>MSLRYIVALTGGIGSGKSTVANAFADLGINVIDADIIARQVVEPGAPALHAIADHFGANMIAADGTLQRRALRERIFANPEEKNWLNALLHPLIQQETQHQIQQATSPYVLWVVPLLVENSLYKKANRVLVVDVSPETQLKRTMQRDDVTREHVEQ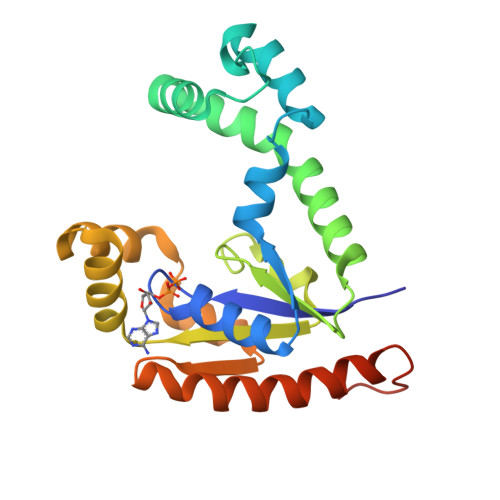ILAAQATREARLAVADDVIDNNGAPDAIASDVARLHAHYLQLASQFVSQEKPEGGSHHHHHH[3x]(4-CARBAMIMIDOYLPHENYL)-METHYL-PHOSPHINIC ACID 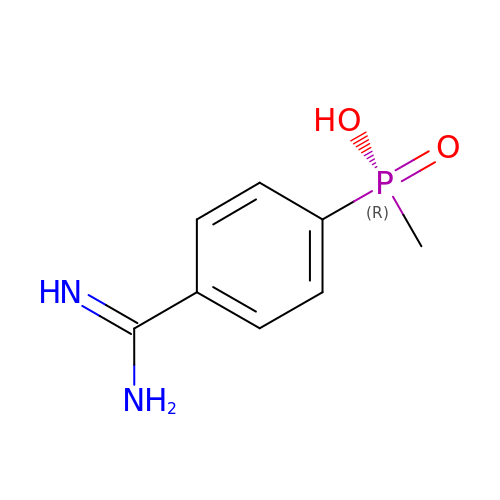| C8 H11 N2 O2 P | CVABPMXIKVDCLF-UHFFFAOYSA-N> MGSSKPLKGFVICCTSIDLKQRTEISTKATKLGAAYRSDFTKDVTHLIAGDFDTPKYKFAAKSRPDIKIMSSEWIPVLYESWVQGEDLDDGLLVDKHFLPTLFKCRVCLTNIGQPERSRIENYVLKHGGTFCPDLTRDVTHLIAGTSSGRKYEYALKWKINVVCVEWLWQSIQRNAVLEPQYFQLD;> GVMTVPNTPQKPNLQ

TOPBP1 and its fission and budding yeast orthologues Rad4 and Dpb11, respectively, are scaffold proteins that mediate formation of multi-protein complexes in a range of essential DNA replication and repair processes. Bioinformatic analysis suggests that only three of the BRCT domains in the yeast TOPBP1 homologues, and four in the vertebrate TOPBP1 homologues, possess the required cluster of residues needed to bind phosphorylated peptide motifs. Despite the structural similarity of these phosphopeptide-binding BRCT domains, genetic and biochemical studies show that they are nonetheless selective and specific for the phosphopeptide sequences with which they interact. To gain some insight into this, we have determined crystal structures of segments of yeast and vertebrate TOPBP1 that contain the two most N-terminal phosphopeptide binding sites (BRCT1 and BRCT2), in complex with phosphopeptides derived from a number of different known ligand proteins, including RAD9, and used this to develop consensus patterns that encapsulate the individual specificity requirements of these two independent binding sites.

Mbd1 is the S. pombe orthologue of the metazoan DNA damage mediator protein MDC1 and plays important roles in the DNA damage response. To try and identify other potential phosphorylation sites on Mdb1 that might mediate its interaction with Rad4, we searched the Mdb1 sequence using ScanProsite as before and identified a good match to the motifs defined above, centred at a documented site of phosphorylation on Thr113. The sequence around Mdb1-Thr113 matches the TP/SP proline-directed kinase consensus and hydrophobic −3 residue seen for many TOPBP1/Rad4 BRCT1 and/or BRCT2 interacting sites. However, based on the presence of a polar residue, threonine at −4 our model would suggest that this site would not display high-affinity for BRCT1. We found that the Mbd1-pT113 peptide bound to Rad4-BRCT1,2 with low micromolar affinity but showed no binding to Rad4-BRCT3,4, the equivalent of TOPBP1-BRCT4,5 that has been implicated in mediating MDC1 interactions in the metazoan system. To determine which BRCT domains mediate the interaction with Mdb1-pT133, we measured binding to Rad4-BRCT1,2 with mutations in BRCT1 (K56E) or BRCT2 (K155E), and found binding was substantially reduced compared to wild-type with the BRCT2 mutant, but was largely unaffected by mutation of BRCT1. Based on these observations, we were able to obtain a high-resolution crystal structure of Rad4-BRCT1,2 in complex with the Mdb1-pT113 peptide, confirming the preference for binding to BRCT2. The structure shows the Mdb1 peptide bound in a very similar conformation as Crb2-pT187, Crb2-pT235 and Sld3-pT650 peptides bound to this domain, with the valine at −3 relative to the phospho-threonine packed into the hydrophobic recess, while the polar threonine at −4 that makes the sequence incompatible with BRCT1, is directed out to solvent by the β-sheet conformation of the peptide backbone.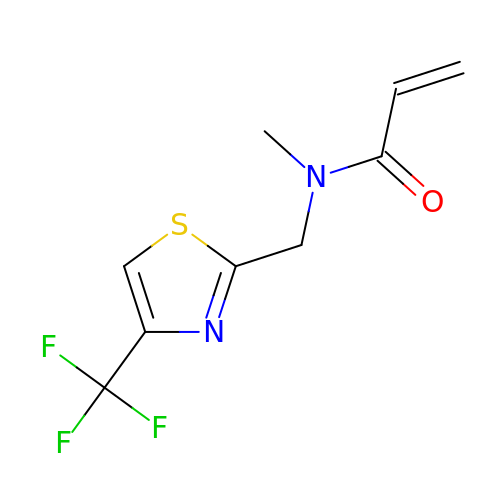N-methyl-N-[[4-(trifluoromethyl)-1,3-thiazol-2-yl]methyl]prop-2-enamide | C9 H9 F3 N2 O S | ZPJNBQRFMJDXHX-UHFFFAOYSA-N> MSEDPILTGVA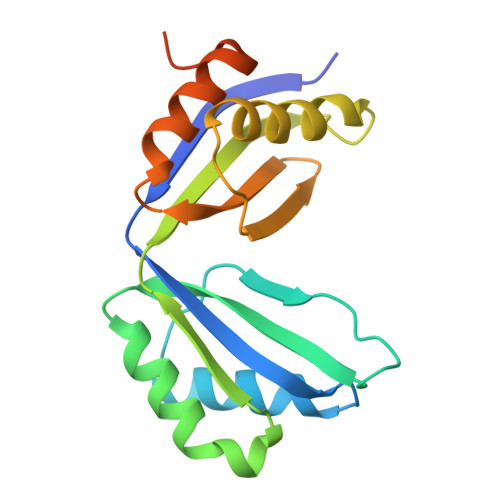HDRSEAKVTIVGLPDIPGYAAKVFRAVADADVNIDMVLQNVSKVEDGKTDITFTCSRDVGPAAVEKLDSLRNEIGFSQLLYDDHIGKVSLIGAGMRSHPGVTATFCEALAAVGVNIELISTSEIRISVLCRDTELDKAVVALHEAFGLGGDEEATVYAGTGRLEHHHHHH2-AMINO-5,6-DIMERCAPTO-7-METHYL-3,7,8A,9-TETRAHYDRO-8-OXA-1,3,9,10-TETRAAZA-ANTHRACEN-4-ONE 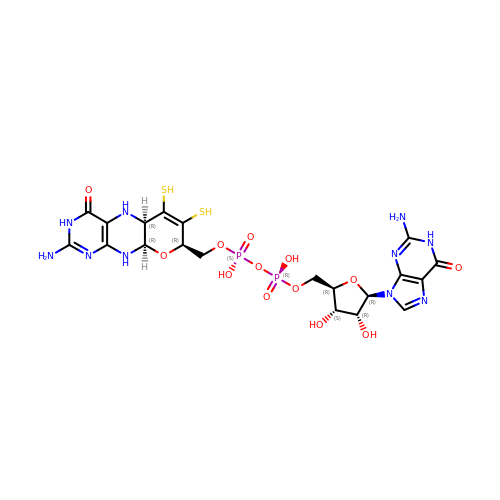GUANOSINE DINUCLEOTIDE | C20 H26 N10 O13 P2 S2 | VQAGYJCYOLHZDH-ILXWUORBSA-N>[2x]MSKPQPIAAANWKCNGSQQSLSELIDLFNSTSINHDVQCVVASTSSHL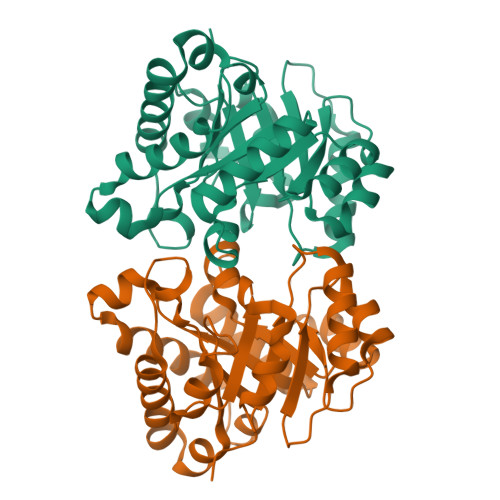AMTKERLSHPKFVIAAQNAGNADALASLKDFGVNWIVLGHSERRAYYGETNEIVADKVAAAVASGFMVIACIGETLQERESGRTAVVVLTQIAAIAKKLKKADWAKVVIAYEPVWAIGTGKVATPQQAQEAHALIRSWVSSKIGADVAGELRILYGGSVNGKNARTLYQQRDVNGFLVGGASLKPEFVDIIKATQ>[4x]TRDQNGTWEMESNENFEGYMKALDIDFCTRKIAVRLTQTKVIDQD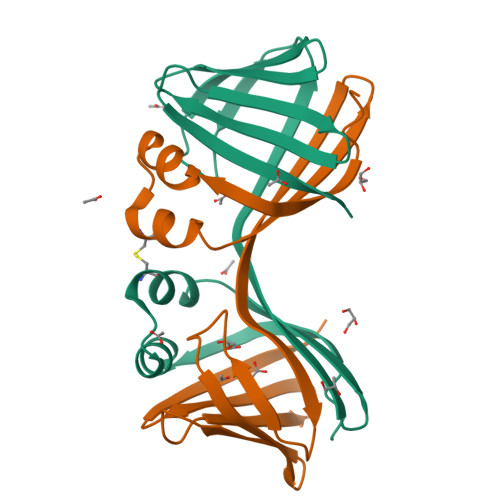GDNFKDKTTSTFRNYDVDFTVGVEFDEYTKSLDNRHVKALVTWEGDVLVCVQKGEKENRGWKKWIEGDKLYLELTCGDQVCRQVFKKK>GAGAGSKRIQLEPLPPLTPKFLNILDQVCIQCYKDFSPTIIEDQAREHIRQNLESFIRQDFPGTKLSLFGSSKNGFGFKQSDLAVCMTINGLETAEGLDCVRTIEELARVLRKHSGLRNILPITTAKVPIVKFFHLRSGLEVDISLYNTLALHNTRLLSAYSAIDPRVKYLCYTMKVFTKMCDIGDASRGSLSSYAYTLMVLYFLQQRNPPVIPVLQEIYKGEKKPEIFVDGWNIYFFDQIDELPTYWSECGKNTESVGQLWLGLLRFYTEEFDFKEHVISIRRKSLLTTFKKQWTSKYIVIEDPFDLNHNLGAGLSRKM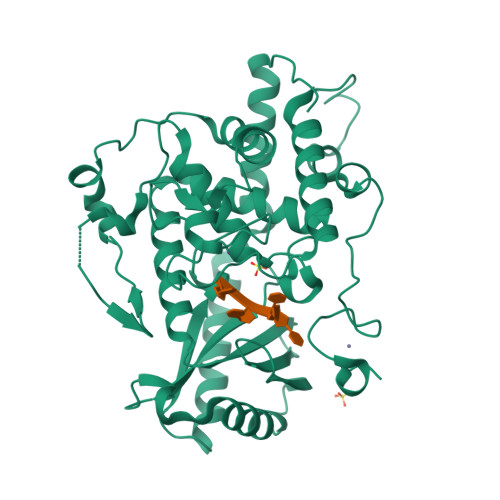TNFIMKAFINGRRVFGIPVKGFPKDYPSKMEYFFDPDVLTEGELAPNDRCCRICGKIGHFMKDCPMRRK[3x]> MPAVASVPKELYLSSSLKDLNKKTEV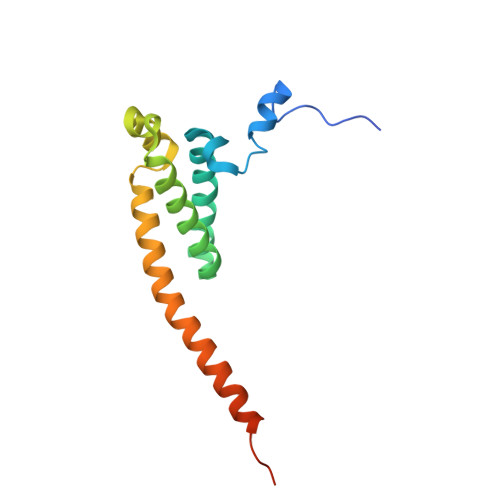KPEKISTKSYVHSALKIFKTAEECRLDRDEERAYVLYMKYVTVYNLIKKRPDFKQQQDYFHSILGPGNIKKAVEEAERLSESLKLRYEEAEVRKKLEEKDRQEEAQRLQQKRQETG>[24x]MPVPNPTMPVKGAGTTLWVYKGSGDPYANPLSDVDWSRLAKVKDLTPGELTAESYDDSYLDDEDADWTATGQGQKSAGDT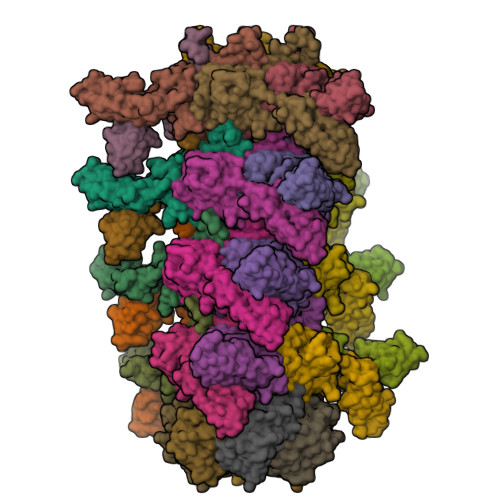SFTLAWMPGEQGQQALLAWFNEGDTRAYKIRFPNGTVDVFRGWVSSIGKAVTAKEVITRTVKVTNVGRPSMAEDRSTVTAATGMTVTPASTSVVKGQSTTLTVAFQPEGVTDKSFRAVSADKTKATVSVSGMTITVNGVAAGKVNIPVVSGNGEFAAVAEITVTAS;>MKHTELRAAVLDALEKHDTGATFFDGRPAVFDEADFPAVAVYLTGAEYTGEELDSDTWQAELHIEVFLPAQVPDSELDAWMESRIYPVMSDIPALSDLITSMVASGYDYRRDDDAGLWSSADLTYVITYEM[6x]>[2x]MTADELVFFVNGKKVVEKNADPETTLLAYLRRKLGLRGTKLGCGEGGCGACTVMLSKYDRLQDKIIHFSANACLAPICTLHHVAVTTVEGIGSTKTRLHPVQERIAKSHGSQCGFCTPGIVMSMYTLLRNQPEPTVEEIEDAFQGNLCRCTGYRPILQGFRTFAKNGGCCGGNGNNPNCCMNQKKDHTVTLSPSLFNPEEFMPLDPTQEPIFPPELLRLKDVPPKQLRFEGERVTWIQASTLKELLDLKAQHPEAKLVVGNTEIGIEMKFKNQLFPMIICPAWIPELNAVEHGPEGISFGAACALSSVEKTLLEAVAKLPTQKTEVFRGVLEQLRWFAGKQVKSVASLGGNIITASPISDLNPVFMASGTKLTIVSRGTRRTVPMDHTFFPSYRKTLLGPEEILLSIEIPYSREDEFFSAFKQASRREDDIAKVTCGMRVLFQPGSMQVKELALCYGGMADRTISALKTTQKQLSKFWNEKLLQDVCAGLAEELSLSPDAPGGMIEFRRTLTLSFFFKFYLTVLKKLGKDSKDKCGKLDPTYTSATLLFQKHPPANIQLFQEVPNGQSKEDTVGRPLPHLAAAMQASGEAVYCDDIPRYENELFLRLVTSTRAHAKIKSIDVSEAQKVPGFVCFLSADDIPGSNETGLFNDETVFAKDTVTCVGHIIGAVVADTPEHAERAAHVVKVTYEDLPAIITIEDAIKNNSFYGSELKIEKGDLKKGFSEADNV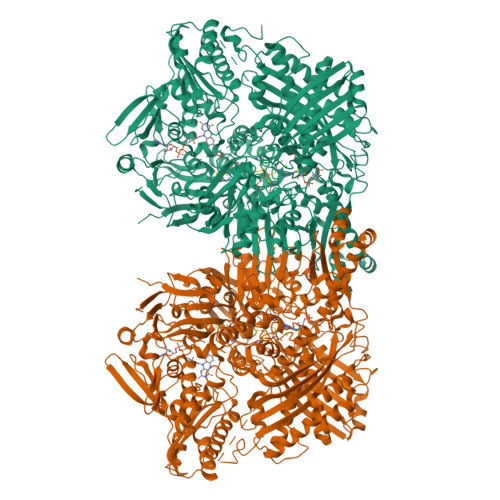VSGELYIGGQDHFYLETHCTIAIPKGEEGEMELFVSTQNAMKTQSFVAKMLGVPVNRILVRVKRMGGGFGGKETRSTLVSVAVALAAYKTGHPVRCMLDRNEDMLITGGRHPFLARYKVGFMKTGTIVALEVDHYSNAGNSRDLSHSIMERALFHMDNCYKIPNIRGTGRLCKTNLSSNTAFRGFGGPQALFIAENWMSEVAVTCGLPAEEVRWKNMYKEGDLTHFNQRLEGFSVPRCWDECLKSSQYYARKSEVDKFNKENCWKKRGLCIIPTKFGISFTVPFLNQAGALIHVYTDGSVLVSHGGTEMGQGLHTKMVQVASKALKIPISKIYISETSTNTVPNSSPTAASVSTDIYGQAVYEACQTILKRLEPFKKKNPDGSWEDWVMAAYQDRVSLSTTGFYRTPNLGYSFETNSGNAFHYFTYGVACSEVEIDCLTGDHKNLRTDIVMDVGSSLNPAIDIGQVEGAFVQGLGLFTLEELHYSPEGSLHTRGPSTYKIPAFGSIPTEFRVSLLRDCPNKKAIYASKAVGEPPLFLGASVFFAIKDAIRAARAQHTNNNTKELFRLDSPATPEKIRNACVDKFTTLCVTGAPGNCKPWSLRV> AGPVTWVMMIA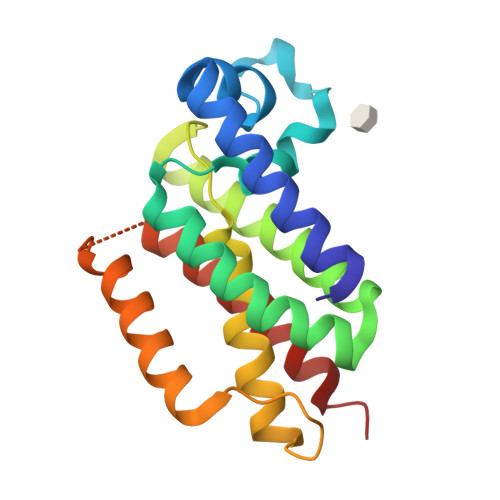CVVVFIAMQILGDQEVMLWLAWPFDPTLKFEFWRYFTHALMHFSLMHILFNLLWWWYLGGAVEKRLGSGKLIVITLISALLSGYVQQKFSGPWFGGLSGVVYALMGYVWLRGERDPQSGIYLQRGLIIFALIWIVAGWFDLFGMSMANGAHIAGLAVGLAMAFVDSLNA>AMYEKPPVEKLIEELRQLKEKAYKGGGDERIQFQHSKGKLTARERLALLFDDGKFNEIMTFATTRATEFGLDKQRFYGDGVVTGWGKVDGRTVFAYAQDFTVLGGSLGETHANKIVRAYELALKVGAPVVGINDSGGARIQEGALSLEGYGAVFKMNVMASGVIPQITIMAGPAAGGAVYSPALTDFIIMIKGDAYYMFVTGPEITKVVLGEEVSFQDLGGAVVHATKSGVVHFMVDSEQEAINLTKRLLSYLPSNNMEEPPYIDTGDPADRDATGVEQIVPNDAAKPYNMREIIYKIVDNGEFLEVHKHWAQNIIVGFARIAGNVVGIVANNPEEFGGSIDIDAADKAARFIRFCDAFNIPLISLVDTPGYVPGTDQEYKGIIRHGAKMLYAFAEATVPKITVIVRKSYGGAHIAMSIKSLGADLVYAWPTAEIAVTGPEGAVRILYRKEIQQASNP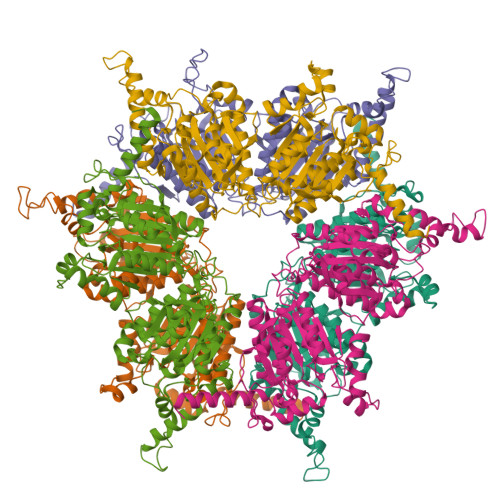DDVLKQRIAEYRKLFANPYWAAEKGLVDDVIEPKDTRRVIVAGLEMLKTKREYRYPKKHGNIPL[6x]> HMEAVLYSTFRNHLKDYMKKVNDEFEPLTVVNKNPDEDIVVLSKSEWDSIQETLRIAQN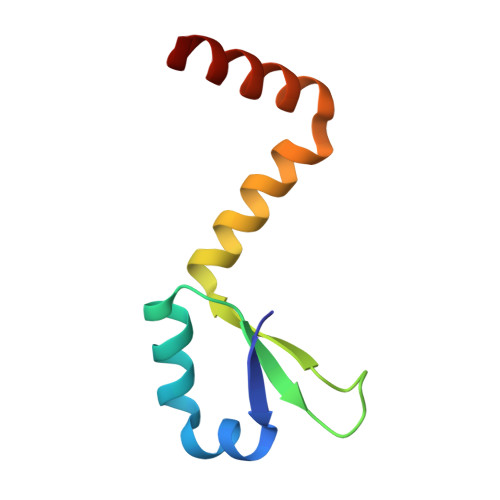KELSDKVLRGMAQVRA> SSGSKSSNSSAKKSAGKPQQGGDLVVGSIGEPTLF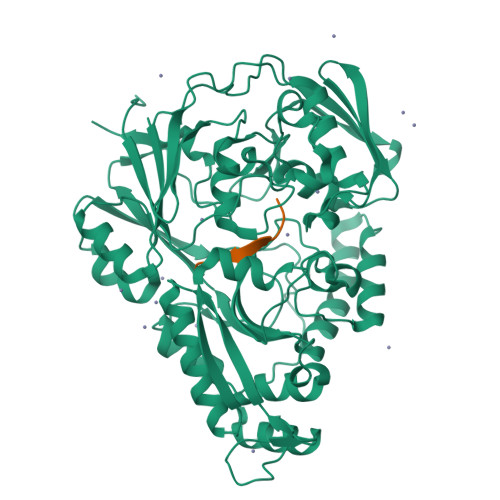NSLYSTDDASTDIENMLYSFLTKTDEKLNVKLSLAESIKELDGGLAYDVKIKKGVKFHDGKELTADDVVFTYSVPLSKDYKGERGSTYEMLKSVEKKGDYEVLFKLKYKDGNFYNNALDSTAILPKHILGNVPIADLEENEFNRKKPIGSGPFKFKEWKQGQYIKLEANDDYFEGRPYLDTVTYKVIPDANAAEAQLQAGDINFFNVPATDYKTAEKFNNLKIVTDLALSYVYIGWNEKNELFKDKKVRQALTTALDRESIVSQVLDGDGEVAYIPESPLSWNYPKDIDVPKFEYNEKKAKQMLAEAGWKDTNGDGILDKDGKKFSFTLKTNQGNKVREDIAVVVQEQLKKIGIEVKTQIVEWSALVEQMNPPNWDFDAMVMGWSLSTFPDQYDIFHSSQIKKGLNYVWYKNAEADKLMKDAKSISDRKQYSKEYEQIYQKIAEDQPYTFLYYPNNHMAMPENLEGYKYHPKRDLYNIEKWWLAK;> VDSKNTSSW> ARTKQT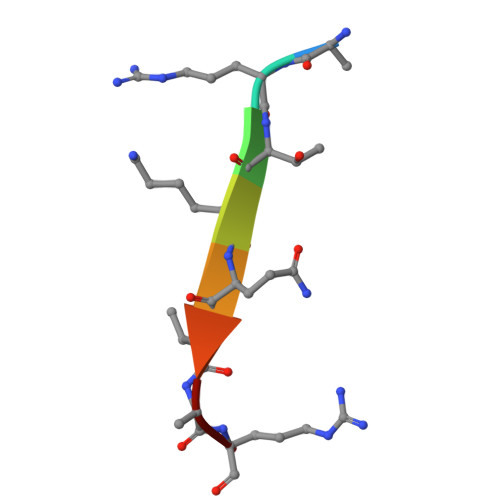AR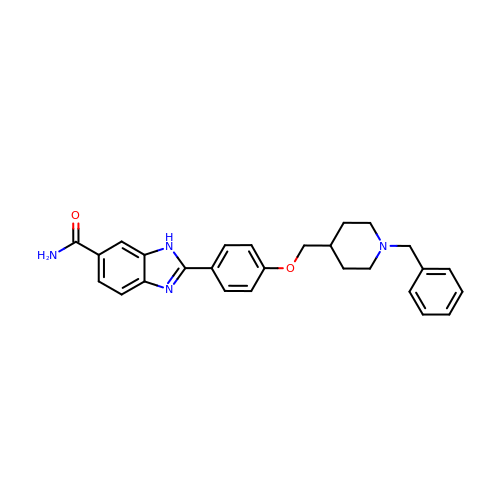2-{4-[(1-BENZYLPIPERIDIN-4-YL)METHOXY]PHENYL}-1H-BENZIMIDAZOLE-6-CARBOXAMIDE | C27 H28 N4 O2 | LTUJRTNXSJGLBT-UHFFFAOYSA-N> ESLVCNLRQLKCHFTWNLIAEDESLDEFEDRVFNKDEFQNSEFKATMCNILAYVKHCRGLNEAALQCLGEAEGFIQQQHPDQVEIRSLVTWGNYAWVYYHMGQFSKAQAYLDKVKQVCKKFSSPYRIENPALDCEEGWARLKCTKNQNERVKVCFQKALEKDPKNPEFTSGWAIANYRLDDWPARNYCIDSLEQAIQLSPDNTYVKVLLALKLDAVHKNQAMALVEEALKKDPSAIDTLLRAARFYCKVYDTDRAIQLLRKALEKLPNNAYVHYYMGCCYRSKVHHMLNRREMVFSGDRKKLEELIQLAVNHLRKAE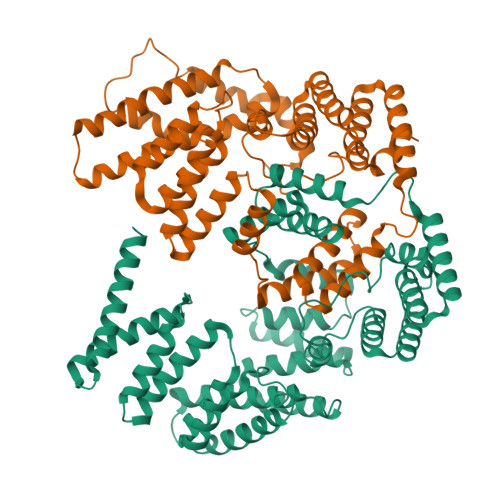EIKEMLEYSCSFLADLYIIAKKYDEADYYFQKELSKDLPPGPKQLLHLRYGNFQFFQMKRQDKAIYHYMEGVKIKKKTIPQKKMREKLQRIALRRLHEDESDSEALHILAFLQENGGGQQADK;> SLEAILPQLKCHFTWNLFREGSMSSHMEDRVCNQVEHLNSEEKATMYDLLAYIKHLDGESKAALECLGQAEDLRKSEHNDQSEIRRLVTWGNYAWIYYHMGRLSEAQAYVDKVRQVCQKFANPYSMECPELECEEGWTRLKCGRNERAKMCFEKALEEKPKDPECSSGMAIAMFRLEEKPEKQFSVDALKQAMELNPQNQYLKVLLALKLLRMGEEAEGERLIKDALGKAPNQTDVLQKAAQFYKKKGNLDRAIELLGKALRSTVNNSPLYSLVMCRYREILEQLQNKGDADSSERRQRMAELRRLTMEFMQKTLQRRRSPLNSYSDLIDFPEVERCYQMVISKESPDVEEEDLYERYCNLQEYHRKSEDLAALECLLQFPR> IDPFTMKKIFMMVHELDVNKGGMTSSMFNRSKEFYDADIPADIVTFDYKGNYDEIIKALKKQGKMDRRTKMYNVFEYFKQISNNKHFKSNKLLYKHISERLKNTIEIEESKGISRYFDITTGTYIAYIRKSKSEKVIDFFKDNKRIERFSFIDNKVHMKETFNVDNKVCYQVFYDEKGYPYISRNINANNGAVGK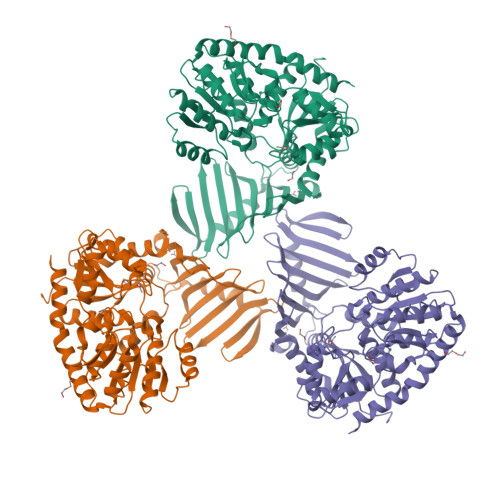TYVLVNKKEFKNNLALCVYYLEKLIKDSKDSIMICDGPGSFPKMFNTNHKNAQKYGVIHVNHHENFDDTGAFKKSEKYIIENANKINGVIVLTEAQRLDILNQFDVENIFTISNFVKIHNAPKHFQTEKIVGHISRMVPTKRIDLLIEVAELVVKKDNAVKFHIYGEGSVKDKIAKMIEDKNLERNVFLKGYTTTPQKCLEDFKLVVSTSQYEGQGLSMIEAMISKRPVVAFDIKYGPSDFIEDNKNGYLIENHNINDMADKILQLVNNDVLAAEFGSKARENIIEKYSTESILEKWLNLFNS> MFTRRGDQGETDLANRARVGKDSPVVEVQGTIDELNSFIGYALVLSRWDDIRNDLFRIQNDLFVLGE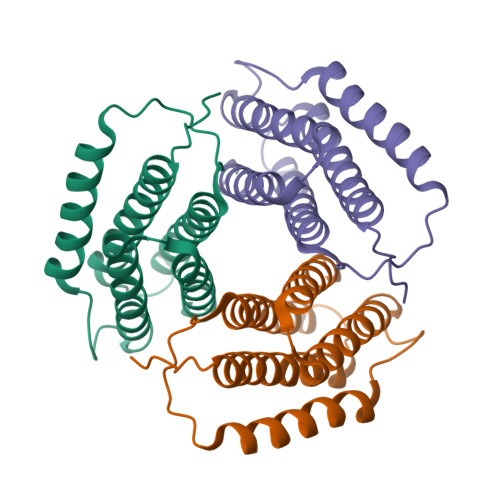DVSTGGKGRTVTREMIDYLEARVKEMKAEIGKIELFVVPGGSVESASLHMARAVSRRLERRIVAASKLTEINKNVLIYANRLSSILFMHALISNKRLNIPEKIWSIHRVS> SDNTRTLPDRENSCPGLLLLLLPIMKTAIALLPFLGAATAFVTPMSKTSMARGRSLQMSFDDEAGAIQWFPPSPGYWDPLGFVADGDTEKFSKYRAIEIKHGRVAMLGALDYFIKTPSGWHLPGKLGDVDIDSIPVGLGAIKAVPPLGWVQIL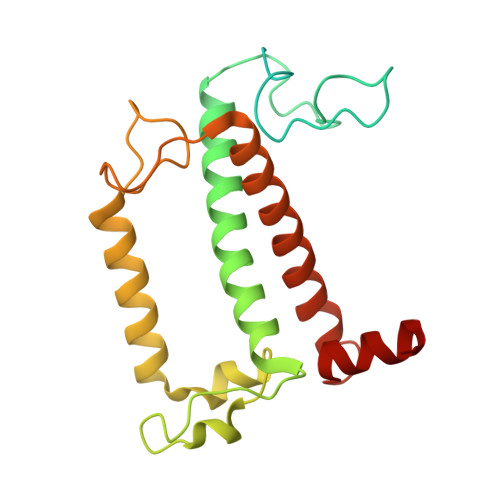LFASALEFLAPQKEDQPPGAVQPATPSFEQPGTLEYQTKEINNGRLAMIALAGLWLGELASGGTDPIVAFKTWVGI> MADSPNRLNRAKIDSTTMKDPRVLNNLKLRELLLPKFTSLWEIQTEVTVDNRTILLTWMHLLCESFELDKSVFPLSVSILDRYLCKKQGTKKTLQKIGAACVLIGSKIRTVKPMTVSKLTYLSCDCFTNLELINQEKDILEALKWDTEAVLATDFLIPLCNALKIPEDLWPQLYEAASTTICKALIQPNIALLSPGLICAGGLLTTIETDNTNCRPWTCYLEDLSSILNFSTNTVRTVKDQVSEAFSLYDLEIL;> MEKDGLCRADQQYECVAEIGEGAYGK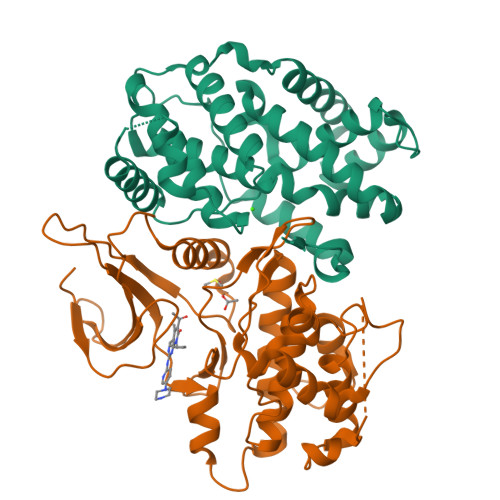VFKARDLKNGGRFVALKRVRVQTGEEGMPLSTIREVAVLRHLETFEHPNVVRLFDVCTVSRTDRETKLTLVFEHVDQDLTTYLDKVPEPGVPTETIKDMMFQLLRGLDFLHSHRVVHRDLKPQNILVTSSGQIKLADFGLARIYSFQMALTSVVVTLWYRAPEVLLQSSYATPVDLWSVGCIFAEMFRRKPLFRGSSDVDQLGKILDVIGLPGEEDWPRDVALPRQAFHSKSAQPIEKFVTDIDELGKDLLLKCLTFNPAKRISAYSALSHPYFQDLERCKE> MLSSKYSKRIAWMKTTICDSLQLKDMIVEESFQYEKNKNLLEQFLSGEGLNKIFAYYQVQEQAQNDDIKDTGAQDPVLFFTTGDLEKIQDKAVWFLRITNPADDKKKASQQDGNDNDIIFGEITPNTVPMLNALMESVYSRQIDHIITEKIQFWGVAEEEQVLEFQQHSNKFSSEVREAINLMSPGTEHFKLDYEAISGLSESEKMQHYEMKFNEWINLISSQLNDDSEVRKDEKDAGPATELIYWRSRMQKITNWSEQLKSKDFQIVKASLQRHKNHDNQRPRGDESLSKLMMEYNRLDLLLTDKLNEAKDNVKYLTTLEKFIEPLYNGTPQQIIDTLPALMNAIKMIHTIARFYNTTDKMTGLFIKITNQMIKNCKDRILNKKDNGDNPSLYKMIWEQDPAELIEVLGSCIKLYCEYKKCYNDTKEKVADMPKGKTFDFSDAQIFGKFDTFVRRLQKLIEIFSNIQQFNALAKHNLEGMDVLTNKFKKIIDDFKKKGHNLLDTANNKFDRDWVEFNVEISHLDGELQNFIDNNFNRFRNIEYSLKLLHKFQSTIKRDSLKHNLTSRYNAILHNYATELDTIQRVFQDQKSNPPLVRNMPPEAGKIIWARHLFQKITGPINIFPENVINSTEIRRYYGSYNTLGKQLTIYEMWFYQDWVNKIEQSKAALQATLIVRHDENKKLYVNFDLEIMQLIREAKCLDRQGIEIPESARIILLQEDKFKTYYNELLYALKEYERINSKIKPICKNLLLPHIEDLDLKLRPGMVTLTWTSMNIESYLYYVHQGLKKLEQLIINVNDIIENRIENNLKTVSKVVLVHLPQDTKPLSLDSFVQLQEEYINSKTDFLTSKNVEVERAVDDLLQTIMLYPLDPHVDPVLPEETKRIKRYYFWYFYQALLNSTQNSLNAMKYRVCGKKIPGANTLQNLKPFFQVEVQLNGDKVTLNPSLQEIQKSINRAATAVLRCSKHLYNWDQQNKDSTDKATFYDMIACDKEIVKVILLLTGSIQGTKNKVNEFLSGFTKFEWLCKESIQESIKKFSKNGPTLQNYEDQLKKFSQIEEEIEKIVPTYKIGAMELMTHNICTSLSTWAKEWKLQYSQDLHKRARQLLDSLTEQTKMLSTKLSKPVKDIDSLGYVMETLEQIRKEQAEIDMKFNPVQEMYSLLDNYLPGGITDKDEMDARSLLRRNWDILIQQAEIKGKEYQHKQAIYLKELKQSIKDFTNQVSIFRRDYEKNGPMVEGISPAEAMERLRRFEDEYDVKYQMYKINARGENLFGLQNQKYPELEKTDAEIKNLNKLYNLYDSVIKNIQQFKEKSWQDVSKDDLAKMEEDAGKYGEQCSRLPKDLKEWQAYRDLKNYIDSLREQLPLIISLKKPSIMPRHWEKIKEITNTKLNYENPDQFYIEEIMGAKLLDFREDIEDITESADKQLKIRTGLDEINLYWNDMQFQFGIWGKRDVPCMLNGLIVGTILERLEEDQLQLSTFNSQRHVTPFKAEVENLIRTFSDVNDTLDMWVKVQKLWTSLEPVFTGGDIARQMPLQAKQFQGIDKNWMKIMEKAVETKKVIPCCQNDMLKDFLPDLNRKLEDCQKMLEAYLEGKRKKFPRFYFVSNPTLLKILSQGSEPTSIQEDFEKLFDAITKVTFESAKDKKNPALKQITQIQQVIGRNEENISLTGYYVKCEGNIEDWLKKLEQNMQQTLKDIASAAAQQVFQVGLKEFVSSQASQIALLGLQILWTSKVNEGLERLSRNERNAMDIKRNEIKEHMNILSSMCLEDLNGAVERTKVETLVTIQVHQKDISMDLKCKDVNDFEWQKQTRIAWKTDIDECIISITDWDSPYSYEFLGAKERLCITPLTDRCYITLAQAMSMYYGGAPAGPAGTGKTETVKDLGRTLGVFVVVTNCSDQHRYRDMAKIFKGLVQSGLWGCFDEFNRIDLEVLSVVAMQVESITTARKQHMKKFMFPEEEIEIELIPTVSYFITMNPGYAGRQELPENLKVLFRGVSMMVPDREIIIKVKLASVGYLQIDLLAKKFNVLYRLCEEQLSKQRHYDFGLRNILSVLRTAGNTKRQEIKSDEEMLLMRSLRDMNLSKLVADDIPLFNGLLADIFPKLKEVPKKLYPDVEKKIPEEINAESYLINTPSFQLKIIQLYETCLVRHGFMLVGPTGSGKSTIMKILTEVLTKLGSPHKIVIMNPKAITAEQMYGVKSEISDDWIPGVFSTIWAKSNNRALKHTTWITCDGPVDAIWIENLNTVLDDNKILTLANGERIAMTENCKVVFEVENLNNASPATVSRCGQVYVSPTDLGYEAVIEGWIRNRKASGRAEESDKLGNILRKYLINMRFIELQSKECKEPMMDTSPVISVINILNLLTGCLQYFVQTQRTLSEQEYEKFIVYSMAWAIGGIYEAQDRVRFHELLLAKNAPIPQKGKENETVFDYYVSQDYLDWKICSPEEWVPPQSLQFSQLLLPTLDSFRAEMLLNFILTQPKSHTCSNSALLIGGSGTAKTSSVLLYCNKFDPQKMLFKRTNFSSATSPFMFQSTIEAECDFKVGKEFAPPGNKMMTIFIDDMSMPFVNKWGDQITLELVRQLIETGGFYMLDKTQRGNQRKMKNLQYIGAMNHPGGGRNDIPNRLKRQFFIFNMILPLSIEGIYGPIIKHMFKQKYFSDSTYKVIESLTSATIALWNKVKSTMLPTPAKFHYVFNMRELSRIFKGILTCKKDTINDAPKSMKIKPELFLVGLWRHEAERVLADKLVNNKDKDTVMGYIQEVSLESFSQIENEILEKYSSEKTFLFCDFLRPDVINEDGIIEEEAPKIYEAIDSLTELRKRCNFLLSFYNDRNPSKKMPLVLFDDALKHLLRISRIIRQPRSSGLLVGVGGSGKQSLTRLAGFIGKNLIQQIIVTKTYSDKDLKEDIKKGFDDAGHLGKQVTFLMTDSEVKKEEFLEYINMVLSTGEIPNLLAKDEREVWLGDISQAYCKEKNLGNIDPPQSELWTYFVDRVRDNFHIMLCFSPVGQKFRERARKFPALFNECTIDWFLPWPEEALVSVAETFIKNFDKLDTKEETKQELMKHMGNVHLMVNEICDEYYQKMRRQVYVTPKSFLSYLNSYKTLYIEKYDELDQQEESFKIGLNKIQEATITINQMEISLKEEEIQLNEATEKTNQLLANLDKESKKANQKGEEVAATNKQCEIQAEQISKEKEEAERELEAALPALRRAQEAVDSIESKDIVELKANKKPLDIIKYIMDAVLVFFKARLIPIQIEERVFNKKEGKAVLFLKESYDESGIQTLGDMNFMKKLKEFEKDSINEETIELLEPYLNQSEDWFNDTFATKASKAAAGILKWAFAIYEYHQKSKIVKPKRIQVAIAEGRQAIALKELEKAREDLAQIQAYIKNLKDVYTKQMEEKNELEMKAAKTKKKINTARTLITSLSGEKDRWGKGAQDISDQKRKLVGNVSLSTAFISYCGPFNAEYRNKLAQQRFVVDMKKRGVPVTPGLELTSFLIDDATIGEWNLQGLPKDDLSIQNGIMVTNSARYPLFIDPQGQGQNWIRNKLSASIIPERCITTLSHPKFKDMFLKYCMESGLTLIVENIENEVDPMMDPVLERQIIVKGKTQFVNVAGTEMELSKEFKLFMTCRLANPSFSPELSAKTTIIDFTVTQSGLEQQLLGKVISKEQKALEDSLNQLLADVNQNQKDLQRLDKNLLERLINSQGNLLDDTELMDVLNNTKTQAKEVAAKLIDAEIKTKEINEKREQYRPVAIRGSAIYFTMIEVSLVNWMYNSSLEQFLKLFIESIDLSEKAQLPSNRVKNIISFLTFHVYRYVNRGLFEKDKITFILMMAFKILTTAGTISSGDVSLFLKSGDALDIKSERQKQISYLEDNQWLNILALSKHTFSGQTLPFFKELPDLISRSENQWRNWIDKNDPENFPIPDFAESINQEKEIGSFISLCLVRSLRNDRTLIATQNFISNVLGKEFTDPISYPIEGIWQESSNMDPVLFLLSAGADPTSSIDELAKKKKKFPCEKVSMGEGQERVARQVIMKGFVEGGWVILQNCHLGLKFMEEIETLVSPINQIHEDFRLWITCEQHPKFPLGLLQKTLKVTNEPPKGLKAGLYKTFTTIITQEFIDKVDHSNWRSLIFTICFLHSIVIERKKFGPLGWCVPYEYNYSDLEASLLYIEKYLTNLMSTPQPNSHNLPISMNVVRYMICEVQYGGRITDDLDRELFITYGETYLKDGIFGNDYFFYDIMVDGSGQKFKYRIPQNPSAELIKYQEYIAKVPTVDNPEVFGLHSNADLTFRLKESKEMINTVMETRPKDSSVGGGKTREEIVQDKAKDMLKNLPPDYNDVEVRELVSKLGGPNPKTSTERGMTVPLNIFLYQEVTRMQRVIGLVRKTLQDTILAIDGQIIMTPEILEAINAIYDAKVPNSWLYDPSGAEISWLLPNLGSWSTSLSDRNKQLNDWLRSGQRPILFWLTGFFNPQGFLTGMKQEVTRNHKKGDGKGGEAWSLDDVVYSTTVKEREKEKDIEQPPAEGVYIKGLYLEGCKWSKNGLDDSDPKKIFADLPILHVSAINKKKTNEQDRMSNTYLCPVYKYPKRTDKYLIFRVGLPCEGSNNPSHWKLRGVALLCSTE;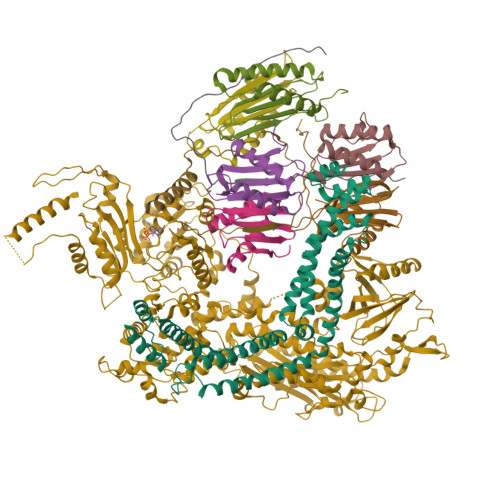> MGDHANEQIIDMPENSEMKSMKNDAFSQAKFAVENYKFENKISSHIKKFFDEKYGPNWHCVVGKHFNAYVSYDSKNFIFFYEGQLAILLYRKG;> MASNQQQKEDPKEQQQQYKTFMGARVLWPPECADDILEGAIRETQDALKKFEIAREGQKIAEHLKKYMDDHFDPYWHVFFGKNFGCQAVHNKNRFIYFYIEKTAFLMYQTQ;> MSDSDSDEGRVVEEPLPPHIIRFNDMAQHLLKKVIRQADVLIKENPQGLEKDIALNLVKFVKSQPEFKIGDGEWQCIIGKNFGCSLTFDANVLAFFDLLPSRKSILLFKSG;> MNHEPEVKATDMEEDMIKRVKEIAINAVKEYKQEKQIAHYIKYEFDKIDGYGWNCIVGRNFGSHIIHQTKKYIFFKINELCLLLWKA;> MKGTYLYLNIYKRKREASLITLNYIKNRFYPSKIQKIIKELFEDRLKGVEYDPNNANQLSERLVLELREKIKRGKVPRYKIGVQVVFGEIKGQGLRIASKCLWDVQNDNYASYTYTSEKVYCTGIVFGCYFE;> MGDTDKEYISEEVQKAIDDSVKQVFGIKDDSSQVTITYNKDKVNLWTQQIIDYTIRGLNKLGKHFKYCVTAILQQTNHAGISVQITAYQDTNTDGSLIQCYEINDIYAIVSVFAMAV;> MFNFFSSANINQNIPKYSVNDFVFRLKKIEKIVVKEGLDGFLLINGVDSRENTEYVKLTNWLFLGNSGLEIEENEYLNQIYSDMIVLIKKGTTHIFIDPEALNSLQTLIYSIPNVDVFCPTEKQYEDKDEMELLKMAFFLRVMKPTKKVGILLGQKDKGKINSIEKWPLIQSYGLEELGVGFFSMNHEVVDLTLRLNAVYKNYDKFFVSKLIYVVAKRLTGHFNSAAGQLGDMKMHKRNLATESQLTEIFRDTYEIEEISKWVQIRGVNAALPKPRVLFGKNTSADCSKEPSVAPLKDLKYSETFHSFHATFETFDLRTCLRAARTYFLAKGVKEERNLITLNDDEGVPQGYELNIDENQQYKDQDFLANLYLSIIIGFNEVMQLITKDYKNMTEEFIQDYIFQKVSKVYAGFQIPESEITLDKIQIILKAYNSFGEEVKIDFKDTISFKLTPYFFMVRIEQKNIKSQILNNTVLGSLVFAESFILQEGCYLLLTKEIPYFDLWNCQNDYSEKIEKMKKRILWEPLGKQISDELPKNRIFVQTGRKSNYGFDIPIMQASYYMHELGLRIETQRLGWFILFFKEMKEIQITQKMNHTWLIFKVDSNITFNSISKDTIALEFTGDALEQSFFKIKNYFEENQIKYEYQVDIPAIFQESQIAKKQILNQQSQGQKLITMNSIQNEQFFISYIESKQLMILNQMKDLKLSAYKNLYEQMQISQAITPVENHIGVILVNGSYCSGKRKFAENLIRFGSDNNLRLHLYKFDLNEMSELTEKSYLSGLLKFASEKKIQNTDVIVASVPHFINTKILIDYFSKSEKISNAFYIRTIATKININNIYSNFNKNPVNNVFTYGVEGYSQFLLLDTYNNYDADVNALNKTLSGVLPGAKIYKIMNNILNPALAKDILTSITFISEQNNLNRLKYSVQYDLLTSNGPSSVVFIPFKLPILREKIRDLIYKKILQNGNQTLVDTIEAEQKIAEFKELNKNSKDPLMIEIIKLKEKIEIQNAQTSDQAIKIDYVKGILRYDSKLKEGLEEITITPNYFIERTVKGVDAKEFTEELNGVSFKNVKYTGITNSIINDMGFVFAGKNLNKEKLLELLYKLVKPLNKQKLRQRKDLTEEEIVDIQFRNRGEGLENGEFYDGQFWRNIQGLILPHHPKKDEFIEEYLKQEEVRINQINEQLQQEWETWKQVYDKIHLDK;> MPPKQTKVVASRKTVMPISRAGRAQIRRKDSNTQNNMNDQGMEDEEIDQQREGMKNQYEQLTAQELNEDMPSKMLEPKNPQAPKNITVYDYYTRKFKTDELVDQMIVHFSMDGDYIWKESNEYKTQEEIRDTKKALIKEAMRKQESEEPGANHDEEAIKQTLRNKFNYNTRECQTINPSIRERGVSTEPPPSDTICGNITQWEIFDAYYAEIMKDHQIENKKKKEVDQDKKQDQSMYSTSFKRCCKIMERMVVQNDQEDKYHDYRYYWSQGDNLEAGKNEGHLLPIWRFSNEKQRKKNVTSICWNPLYPDLFAVSLGSYDFTKQRMGLICLYSLKNTTHPEYAFNCEAGVMCLDFHPKSAALLAVGLYDGTVLVYDIRNKHKKPIYQSTVRNQKHTDPVWQVKWNPDTSKNYNFYSISSDGRVMNWILMKNKLEPEEVILLRLVGKNEEESTLIGLACGLCFDFNKFEPHIFLVGTEEGKIHKCSRAYSGQYQETYNGHLLAVYKVKWNNFHPRTFISASADWTVRIWDSKYTSQIICFDLSMMVVDAVWAPYSSTVFACATMDKVQVYDLNVDKLNKLAEQKIVKQPKLTNLSFNYKDPILLVGDSHGGVTLVKLSPNLCKSGPEIKQTEDKKAMEEFKNVKIEDYEREKMENLLAVVSKWEREDA;> MAEYFTYSKKRKEFNNPINFQDTETRYGGIQNQVVNINQYVQRNPNFIDLDNIAELSEHSVNTERVKTGDRGMSHKEGGWPGNVDPNEAQETGRFKKRIEKDTSFPQAVKDLKEGVEKCIYQNNQIDLLEEYFEGETSEHVVENLSSKTLMLFKDEKEICKRSVSEISWHPEGPTKVAVSYAIMRFQQMPEKMPTQAYVWDLLNPNSPEIKLMSPSAVTNISYNQKIPDQIGGGCYNGLLAVWDGRKGENPIMISPVENSHYEPVTHFHWLMSKTGSECVTTSTDGKVMWWDTRKFEAGPVEKLNIIEGLGENEEIIGGTALEYNVEAGPSKFLIGTESGSILTANKKLKKPVEITTRYGLDQGRHLGPVYSINRSNQNPKYFLSVGDWSCKIWVEDLKTPIIRTKYHGSYLSDGCWSPTRSGAFFLVRRDGWMDVWDYYYRQNEIAFSHKVSDSPLTCIKINQTGGAYHNSGKLCAIGDQDGTVTILELCDSLYTMQPKEKDIINEMFEREYRKEKNLETIKKQQELAKRQVQKDMGSQKEKWEKKKLEMIETAEASFHENLAKNPVNEEEFNELDSPSEKRKKTNQNQGREQEEQSREEQEASGNFNQQQQQQQEEEQQQEGEQQHHQNQEHQNGQGHENGQEEGEENGEEGNQQENEGQEENEQQQE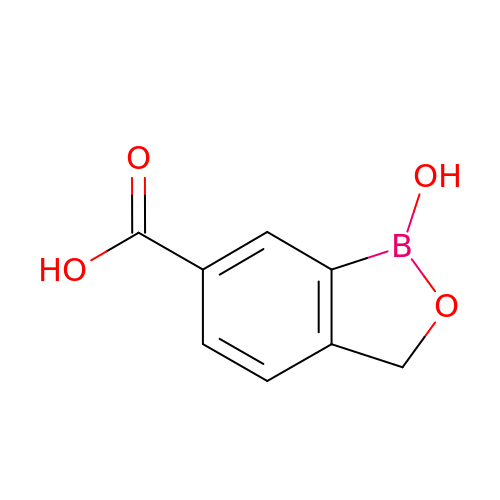1-Hydroxy-1,3-dihydro-2,1-benzoxaborole-6-carboxylic acid | C8 H7 B O4 | VXDGEAYKTHEYPI-UHFFFAOYSA-N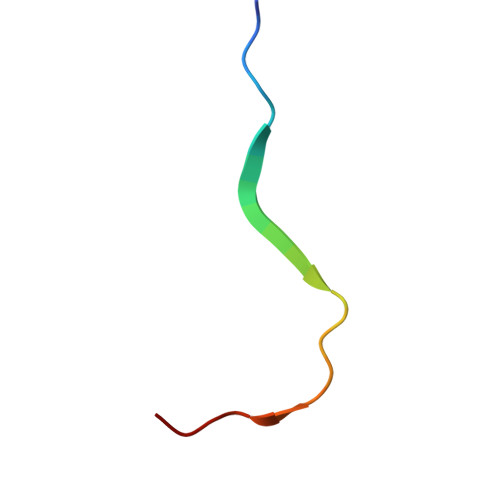> KKGCVVIVGRIVLSGKPAIIPKK> MMMYKEPFGVKVDFETGIIEGAKKSVRRLSDMEGYFVDERAWKEL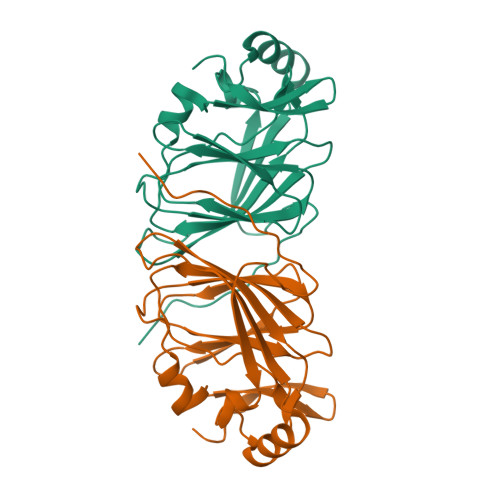VEKEDPVVYEVYAVEQEEKEGDLNFSTHVIYPGKVGKEFFFAKGHFHAKLDRAQVAVALKGKGGVLMQTPEGDAKWISSEPGTVIYSPPYWAARAVNIGDEPFIMLVIYPADAGHDYGTIAEKGFSKIVIEENGEVKVVDNPRWKKGSLEHHHHHH> GLGDELEEVIVEKTKQTVASISSGPKHTQKVPILTANETGATMPVLPSDSIETRTTYMHFNGSETDVECFLGRAACVHVTEIQNKDATGIDNHREAKLF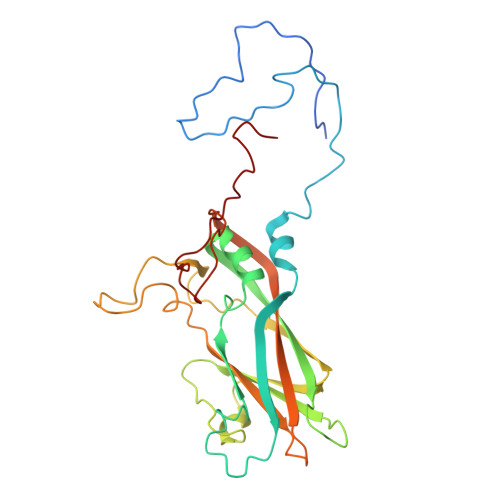NDWKINLSSLVQLRKKLELFTYVRFDSEYTILATASQPDSANYSSNLVVQAMYVPPGAPNPKEWDDYTWQSASNPSVFFKVGDTSRFSVPYVGLASAYNCFYDGYSHDDAETQYGITVLNHMGGMAFRIVNEHDEHKTLVKIRVYHRAKHVEAWIPRAPRALPYTSIGRTNYPKNTEPVIKKRKGDIKSY>SMAEMKAVATSPSGRFLKFDIELGRGAFKTVYKGLDTETWVEVAWCELQDRKLTKAEQQRFKEEAEMLKGLQHPNIVRFYDSWESILKGKKCIVLVTELMTSGTLKTYLKRFKVMKPKVLRSWCRQILKGLQFLHTRTPPIIHRDLKCDNIFITGPTGSVKIGDLGLATLMRTSFA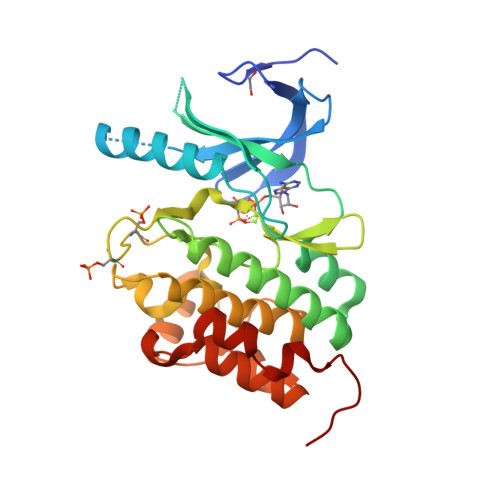KSVIGTPEFMAPEMYEEHYDESVDVYAFGMCMLEMATSEYPYSECQNAAQIYRKVTSGIKPASFNKVTDPEVKEIIEGCIRQNKSERLSIRDLLNHAFFAEDTGLRVE[2x]>[14x]MTDSVQTETTEGKIIINLFAPNLPGSTKEDDLIQKSLRDQLVESIRNSIAYP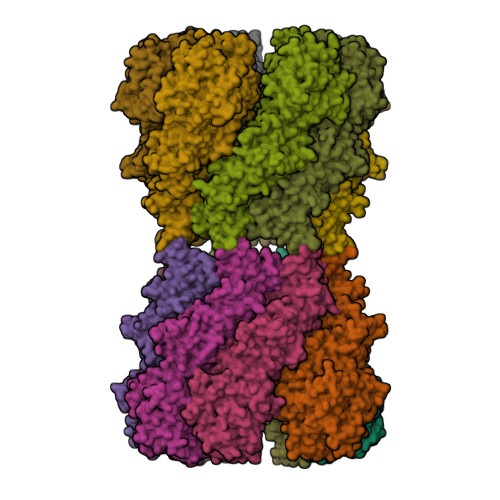DTDKFAGLTRFIDESGRNVFFVDGTRGAGKTTFINSVVKSLNSDQDDVKVNIKCLPTIDPTKLPRHEPILVTVTARLNKMVSDKLKGYWASNDYRKQKEQWQNHLAQLQRGLHLLTDKEYKPEYFSDALKLDAQLDYSIGGQDLSEIFEELVKRACEILDCKAILITFDDIDTQFDAGWDVLESIRKFFNSRKLVVVATGDLRLYSQLIRGKQYENYSKTLLEQEKESVRLAERGYMVEHLEQQYLLKLFPVQKRIQLKTMLQLVGEKGKAGKEEIKVKTEPGMQDIDAIDVRQAIGDAVREGLNLREGSDADMYVNELLKQPVRLLMQVLQDFYTKKYHATSVKLDGKQSRNERPNELSVPNLLRNALYGSMLSSIYRAGLNYEQHRFGMDSLCKDIFTYVKQDRDFNTGFYLRPQSESEALRNCSIYLASQVSENCQGSLSKFLQMLLVGCGSVSIFNQFVTELARAENDREKFEQLISEYVAYMSVGRIESASHWANRCCAVVANSPNDEKIGVFLGMVQLNRKSRQHMPGGYKKFNIDTENGLAKAAMASSLSTVASNNLMDFCSVFNLIGAIADISACRCERSAITNAFNKVIAQTTCIVPPWSEAAVRAEMKGSSKSADNDAAVLDVDLDPKDDGVIDESQQDDATEFSDAITKVEQWLKNVNEIEIGIRPSALLIGKVWSRFYFNLNNVADQHKTRLYRNAEHGRMASQSNAAKIMRFNVLAFLHAVLVEESLYHSVSDREYIGEGLRLNPVTSVDEFEKKIKIIGEKLKADNKTWKNTHPLFFLLISCPILHPFIFPVGGINCSVKALNKETSFNKLIDEIVGDKLLSDEEWDYLTKNNDQKTNTRQQIFQNTITSLNSSTIVGASYDKDTPARKTKSPLLGDSEEK>[10x]MLKVSK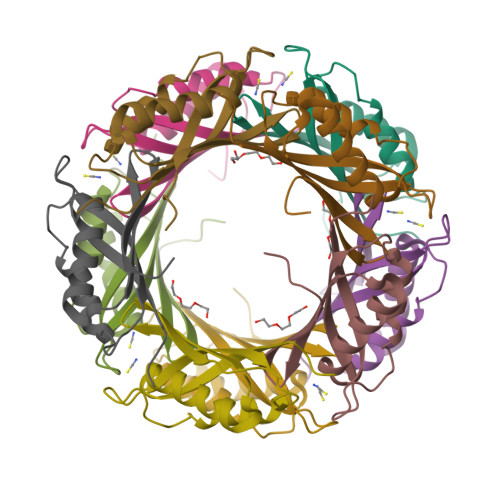SPSLVRLKTRGESVCPISKTVDSFEVSVEYIPRGAVLAIEEFKKMVDSYRGREILHEELAVDLLEKVKAAVNPPYVKVTVKSYYIGVEVEVVAESGGVPPVYI> DGY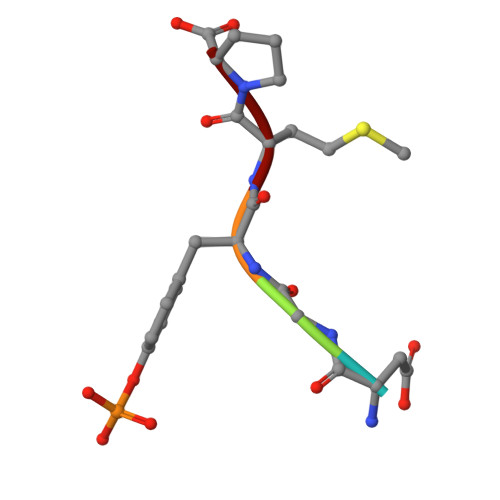MP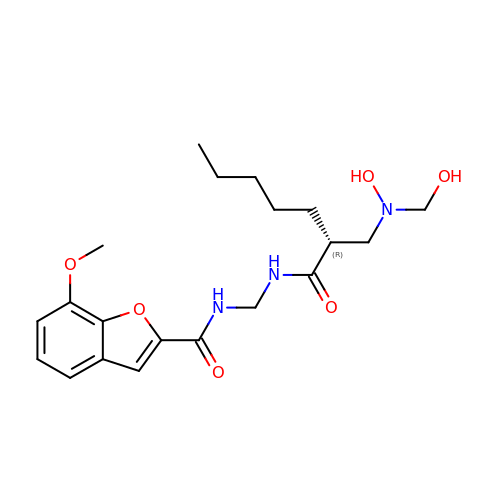N-({[(2R)-2-{[hydroxy(hydroxymethyl)amino]methyl}heptanoyl]amino}methyl)-7-methoxy-1-benzofuran-2-carboxamide | C20 H29 N3 O6 | SHHWEKDWPKWOKJ-OAHLLOKOSA-N Here we report seven high-resolution cryo-EM structures of filamentous peptide nanotubes based on a cross-α supramolecular architecture that provide insight into the designability of helical peptide filaments. A structural interaction is identified based on an appropriately placed pair of arginine residues (RxxxR) within the corresponding peptide sequences. This local interaction motif, designated as an arginine clasp, is robust within the context of these cross-α assemblies and can guide the coalescence of helical protofilaments into structurally defined cross-α nanotubes. In contrast to most structurally characterized filaments based on synthetic α-helical coiled-coils, the chain axes of the helical protomers are oriented in a plane nearly perpendicular to the long axis of the assembly.

Therefore, the designed series of Form I-like peptides encompassed minimal peptide sequences in which the structurally determinative distance between the RxxxR motif and the C-terminus was systematically varied over the range from 2 to 5 heptad repeats. Three filaments, derived from peptides 15-10-3, 29-24-3, and 36-31-3, were selected for further analysis using cryo-EM imaging with direct electron detection. Five protofilaments interacted to form the 15-10-3 filament, four interacted in the 29-24-3 filament, and three interacted in the 36-31-3 filament. In each case, the α-helical protomers within a protofilament stacked along a right-handed n-start helix, in which the value of n corresponded to the number of protofilaments within a nanotube. For example, each 5-start helix of 15-10-3 passed through every fifth protomer and therefore corresponded to the axial stacking direction in a protofilament. For the 29-24-3 peptide, the interaction occurred between the C-terminus of peptide (ia) and the RxxxR motif of peptide (ib + 1), in contrast to the C5-symmetric structure of 15-10-3 that involved helices ia and ib. Despite the differences in cross-sectional geometry for the respective filaments, the helix crossing angles were remarkably similar and lay within the range from 95° to 105°.

>QAEILRAYARILEAQ[105x]> MPLEIRELV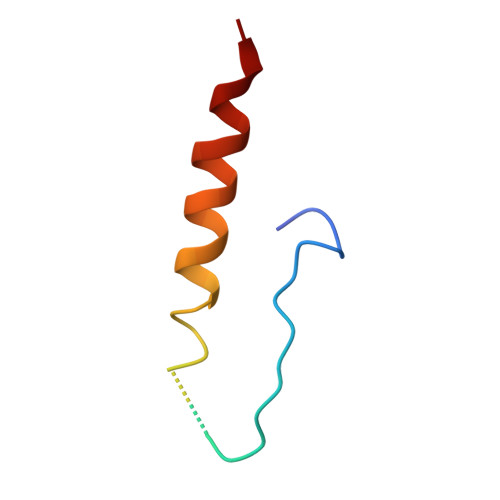IKASVNEGGQNQGTGGAGDQSAIIAACVEQVLAILQEKSER>[2x]SMLNLRYGMETTSLLLCIGNNSSGIRSRHRSYGDASFCYDPVSRKTYFISSPKYGEGLGTVCTGVVMENNTIIVAGEASASKLSRQKNK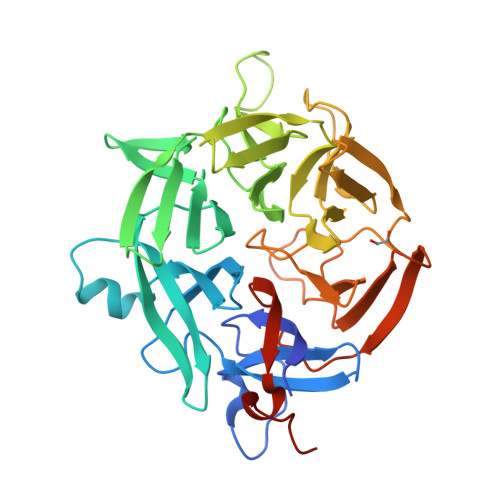NVEIYRYHDRGNQFWEKLCTAEFRELYALGSIHNDLYVIGGQMKIKNQYLITNCVDKYSVERDNWKRVSPLPLQLACHAVVTVNNKLYVIGGWTPQMDLPDEEPDRLSNKLLQYDPSQDQWSVRAPMKYSKYRFSTAVVNSEIYVLGGIGCVGQDKGQVRKCLDVVEIYNPDGDFWREGPPMPSPLLSLRTNSTNAGAVDGKLYVCGGFHGADRHEVISKEILELDPWENQWNVVAINVLMHDSYDVCLVARMNPRDLIPPPSDLVEEGNEHL>ANSKAVCNLPKLAGDETCSNKTEIRWYYNGTACEAFIFKGCGGNDNNFDRVDDCQR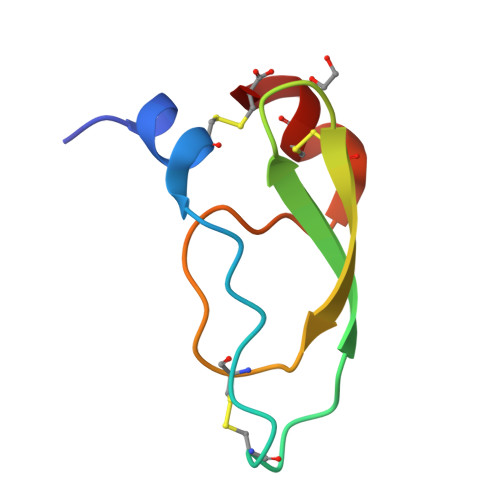LC[2x]BRCC36 is the catalytic subunit responsible for the majority of K63-Ub specific DUB activity in the cytoplasm and in the nucleus as part of two distinct macromolecular assemblies characterized by the presence of either of the MPN− pseudo DUB proteins KIAA0157 or Abraxas. The Abraxas complex (ARISC) functions in DNA repair and breast cancer suppression, while the BRCC36 isopeptidase complex (BRISC) promotes interferon dependent responses by deubiquitinating and stabilizing the type I interferon receptor, IFNAR1. BRCC36 consists of a functional metalloprotease JAMM/MPN+ domain followed by a predicted coiled coil region implicated in protein-protein interactions. KIAA0157 and Abraxas are required for the catalytic function of BRCC36 in both complexes, and enable association of two additional shared subunits (BRCC45 and MERIT40) to each holoenzyme.

Optimization of the CfKIAA0157 construct boundaries by deletion of poorly conserved C-terminal residues 290 to 471 (CfKIAA0157ΔC) yielded crystals in complex with full length CfBRCC36 (residues 1-253) that diffracted to 2.55 Å resolution. Following manual rebuilding and refinement, two highly interdigitated CfBRCC36–KIAA0157ΔC heterodimers were apparent in the asymmetric unit, arranged in the suspected super dimer configuration. The structure of each protomer of CfBRCC36 and CfKIAA0157 consisted of a canonical MPN domain (residues 1–165 in BRCC36 comprising an eight strand β-sheet flanked by three α-helices and residues 1–180 in KIAA0157 comprising a seven strand β-sheet flanked by three α-helices), followed by two non-canonical helices α4 and α5 within the predicted coiled coil regions. The MPN domains of each associated in a pseudo two-fold manner centered on helices α1, resulting in a unified β-sheet and “fused” MPN+–MPN− superstructure (buried SA = 2902 Å2). Non-canonical helices α4 and α5 of CfBRCC36 interacted with helices α4 and α5 of CfKIAA0157 in the form of a coiled coil helical bundle (CCHB). The helical bundle was tethered against the fused MPN domains of BRCC36 and KIAA0157 via a mixture of hydrophobic and hydrophilic interactions.

>GAMDDSSLQKVELQTDVYMVCLQHALSTENFEVMGLLIGNFACGIAKISAVIILRRLDKKKDRVEISSEQLLKAAAEAERLTVELNRPMRVLGWYQSQPHITVCPSHVDVRTQATYQTMDHSFVGLIFSVFSEGKESKEHEIFLNCFQSDNGEATEIPLEIVHTPDISDRCLRTMTDLSKILVQEEEDMAEACKDHPDVLASIHNNAVRTRALIHITDIITKPLVQTFEKRIALNKLRATHLQRQLQELQKMCNG[2x];>[2x]MADSDLLVTISGAALSLLFFENVRSVGNQMGFLLGEALEFIVKTYTDSDNQVETVKIHINVEAIVTCPLADLLHDSTNHINKEKLKDFVRDKSKQVIGWFCFRRNTTNLTLTLKDKLLHKQFASHFSGVNGCKEDFFLTCLLNASTSETSGTHKFRHVFLRHNKRGMFEPISLKINNLGDDASRHDGSDYKPTPVRKSTRTPDSFTKLIESLNLDVARIDGLDSAMLIQKAAEHHLMSLIPKVCESDLEVAELEKQVHELKIKIATQQLAKRLKINGENCDRISKASKD DITHIANE DIOL | C4 H8 O2 S2 | 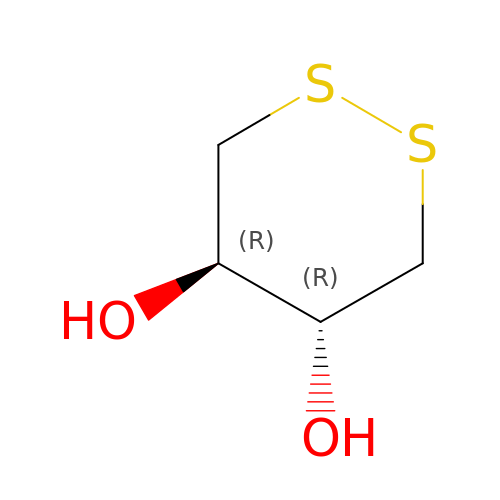YPGMOWHXEQDBBV-IMJSIDKUSA-N Uridine phosphorylase (UPP; EC 2.4.2.3) is a ubiquitous enzyme involved in pyrimidine salvage and maintenance of uridine homeostasis. It catalyzes the reversible phosphorolysis of uracil ribosides and analogous compounds to their respective nucleobases and ribose-1-phosphate. Humans possess two isoforms of UPP (hUPP1 & hUPP2) of which hUPP1 is more widely distributed, more abundantly expressed, and better characterized. hUPP1 has been a subject of interest to cancer researchers due to its role in the activation of pyrimidine nucleoside analogues used in chemotherapy, such as 5-fluorouracil (5-FU) and its prodrug, capecitabine. In contrast to expectations, hUPP1 is dimeric, having lost the higher order assembly (trimer-of-dimers) that results in hexameric rings in more primitive UPPs.

In the present study, we have determined the crystallographic structure of hUPP1 at high resolution, both in ligand-free and BAU-bound conformations. Specifically, one of the three pocket arginine residues (Arg64 in hUPP1) is bent away from the anion, leaving only two coordinating guanidinium groups, one from each subunit of the dimer, to bind the substrate. However, in the ligand-free structure of hUPP1 this residue is found to coordinate a sulfate ion from the crystallization liquor at a position 4.4 Å removed from the catalytic phosphate binding pocket. This finding may imply that in the human enzyme this residue has been adapted to ligand recruitment from the cytoplasm rather than ligand binding in the active site. Determination of both ligand-free and BAU-bound forms of hUPP1 allows direct analysis of the conformational changes induced in the enzyme upon substrate binding. To this end, there are only subtle differences in the fold and residue orientation between overlaid monomers of hUPP1. However, there is a dramatic inter-domain motion between monomers leading to 3–5 Å changes in the relative positioning of the loops undergoing the greatest movement. Another implication of the loss of hexameric structure appears to be that the human enzyme possesses greater inter-domain flexibility than its microbial counterparts. However, the 'open' conformation of hUPP1 provides the opportunity to potentially develop a novel class of allosteric inhibitors of this enzyme that lock the protein in a functionally disabled form, with its catalytic residues too separated to lyse substrates.

> MRGSHHHHHHGSPGLQEFMAATGANAEKAESHNDCPVRLLNPNIAKMKEDILYHFNLTTSRHNFPALFGDVKFVCVGGSPSRMKAFIRCVGAELGLDCPGRDYPNICAGTDRYAMYKVGPVLSVSHGMGIPSISIMLHELIKLLYYARCSNVTIIRIGTSGGIGLEPGTVVITEQAVDTCFKAEFEQIVLGKRVIRKTDLNKKLVQELLLCSAELSEFTTVVGNTMCTLDFYEGQGRLDGALCSYTEKDKQAYLEAAYAAGVRNIEMESSVFAAMCSACGLQAAVVCVTLLNRLEGDQISSPRNVLSEYQQRPQRLVSYFIKKKLSKA We created ADDomer, an adenovirus-derived multimeric protein-based self-assembling nanoparticle scaffold engineered to facilitate plug-and-play display of multiple immunogenic epitopes from pathogens. The penton-forming protomer of certain adenovirus serotypes can self-assemble into a symmetric, hollow dodecahedron adopted by 12 pentons comprising altogether 60 protomers, effectively representing a proteinaceous, nonenveloped VLP. The protomer represents a two-domain architecture, with a crown region comprising the VL and RGD loop abutting a jellyroll fold mediating multimerization. The RGD loop contains a conserved tripeptide motif (-RGD-) mediating integrin-based internalization into target cells.

We used cryo–electron microscopy at near-atomic resolution and implemented novel, cost-effective, high-performance cloud computing to reveal architectural features in unprecedented detail. Our structure shows that the plasticity of the RGD loop and VL, essential for antigenic epitope presentation, is maintained in ADDomer. Close inspection of our cryo-EM structure reveals notable differences. The fiber-binding cleft adopts a rearranged conformation, seemingly in between the geometries observed in the crystals of apo- and fiber-bound Ad3 dodecahedron. In our cryo-EM structure, we observed additional density in between the crown and jellyroll domains, juxtaposed to four sulfur-containing amino acids (M131, M138, M458, and C539), consistent with a tetradentate coordination by a metal ion, possibly zinc or iron. We posit that a structural metal ion at this interdomain interface could be important for stabilizing this protein fold. No corresponding density is observed by cryo-EM. Consequently, glutamates E466 do not extend into the cavity, but the corresponding α-helices are slightly shifted in the ADDomer. Rather, in ADDomer, two neighboring protomers engage in hydrogen bonds in the vicinity of the twofold axis, extending from the S61 side chain to the peptide backbone of E59 and vice versa. We did not observe either of these features by cryo-EM and thus wondered about ramifications for ADDomer stability.

>MRRRAVLGGAVVYPEGPPPSYESVMQQQAAMIQPPLEAPFVPPRYLAPTEGRNSIRYSELSPLYDTTKLYLVDNKSADIASLNYQNDHSNFLTTVVQNNDFTPTEASTQTINFDERSRWGGQLKTIMHTNMPNVNEYMFSNKFKARVMVSRKAPEGEFVTVNDGPVNDTYDHKEDILKYEWFEFILPEGNFSATMTIDLMNNAIIDNYLEIGRQNGVLESDIGVKFDTRNFRLGWDPETKLIMPGVYTYEAFHPDIVLLPGCGVDFTESRLSNLLGIRKRHPFQEGFKIMYEDLEGGNIPALLDVTAYEESKKDTTTARETTTLAVAEETSEDVDDDITRGDTYITELEKQKREAAAAEVSRKKELKIQPLEKDSKSRSYNVLEDKINTAYRSWYLSYNYGNPEKGIRSWTLLTTSDVTCGAEQVYWSLPDMMQDPVTFRSTRQVNNYPVVGAELMPVFSKSFYNEQAVYSQQLRQATSLTHVFNRFPENQILIRPPAPTITTVSENVPALTDHGTLPLRSSIRGVQRVTVTDARRRTCPYVYKALGIVAPRVLSSRTF[60x]>GHMTGPTDATAPARCRVCGDTVDEFLDLGRQPLSDRFLTPADTDGEFFYRLAVGRCHACG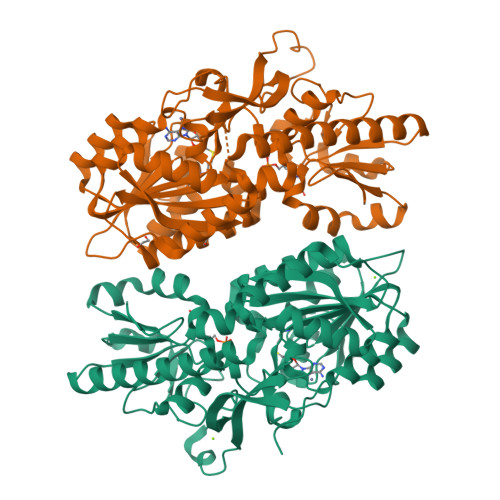MVQLTEEVPRHLMFHEEYPYHSSGSSVMREHFAKVAQRLLATELTGADPFVVEIGCNDGIMLRAVHEAGVRHLGFEPSAGVAEVARSRGVRVRTEFFEKATATAVRESEGPADVIYAANTMCHIPYLESVFQGADALLGPDGVVVFEDPYLGDIVAKTSFDQIYDEHFYLFSAGSVAAMAERFGFELVDVERLPVHGGEVRYTLARRGARTPTEAVGRLLAEEREQGLDDLATLRTFAANVHTVRDELVALLTRLRAEGHRVVGYGATAKSATVTNFCGIGPDLVSFVCDTTPGKQHRLTPGKHLPVRPAEAFADPYPDYALLFAWNHADEIMAKEQEFRQAGGRWILYVPEVRVL[2x]CPB is secreted by C. perfringens type C strains and is essential in the pathogenesis of a lethal necrotic enteritis in many animal species and humans (Uzal et al, 2014). Based on sequence homology between mature CPB and other bacterial toxins, the toxin is a member of the hemolysin‐like family of β‐PFTs. Recently, we determined the molecular basis for the specificity of CPB toward endothelial and leukocytic cells by showing that PECAM‐1/CD31, an endothelial and leukocytic adhesion molecule, serves as its cellular receptor (Bruggisser et al, 2020; Tarek et al, 2021). The cryo‐EM analysis of CPB clearly showed that like other members of the hemolysin‐like family, the CPB protomer is composed of a cap, a rim, and a stem domain (Johnstone et al, 2021).

In the present study, we describe the cryo‐electron microscopy (EM) structure of CPB in SMA discs, which likely represents the membrane‐inserted pore form, at near atomic resolution. Further refinement and postprocessing resulted in an electron density map at an estimated 3.8 Å resolution (and EV2E and F). This allowed us to unambiguously build a model for the CPB octameric pore except for two loops in the rim domain (Glu76–Ser89, Ala283–Pro287), 4N‐terminal amino acids and several amino acids with unresolved side chains. Overall, the CPB octamer forms a 123 Å‐long ring‐like structure with a widest outer diameter of 97 Å. While the N‐terminus of Hla is located inside the cap domain and wraps the vestibule‐exposed surface of the adjacent protomer, the CPB N‐terminus protrudes from the cap as a short hairpin, which assembles to form a 16‐strand β‐barrel. We termed it the N‐terminal β‐barrel protrusion (NBP). It goes through the 25‐Å long N‐terminal ß‐barrel, the central large 72,900 Å3 vestibule, formed by the cap domains, and the transmembrane β‐barrel. The narrowest points have a ~ 6 Å mean radius and are located within the NBP at the level of the positively charged Arg11 and Lys13. The wide cap vestibule features a balanced amount of positive and negative charges, while the transmembrane β‐barrel is overall negatively charged, especially due to Glu152 and Glu162. In conclusion, the CPB pore has a C8 symmetry unlike the C7 symmetries of the homo‐component members of the hemolysin family and similar to the enterococcal EPX toxins.

>NDIGKTTTITRNKTSDGYTIITQNDKQIISYQSVDSSSKNEDGFTASIDARFIDDKYSSEMTTLINLTGFMSSKKEDVIKKYNLHDVTNSTAINFPVRYSISILNESINENVKIVDSIPKNTISQKTVSNTMGYKIGGSIEIEENKPKASIESEYAESSTIEYVQPDFSTIQTDHSTSKASWDTKFTETTRGNYNLKSNNPVYGNEMFMYGRYTNVPATENIIPDYQMSKLITGGLNPNMSVVLTAPNGTEESIIKVKMERERNCYYLNWNGANWVGQVYSRLAFDTPNVDSHIFTFKINWLTHKVTAI[8x]> MGKYNLILSEYLSFIYNSQSAVQIPIYYSSNSELENRCIEFHSKCLENSKNGLSLRKLFVEYNDVIENATLLSILSYSYDKYNAVERKLVKYAKGKPLEADLTVNELDYENNKMTSELFPTAEEYTDSLMDPAILTSLSSNLNAVMFWLEKHENDVAEKLKVYKRRLDLFTIVASTINKYGVPRHNAKYRYEYDVMKDKPYYLVTWANSSIEMLMSVFSHDDYLIAKELIVLSYSNRSTLAKLVSSPMSILVALVDINGTFITNEELELEFSNKYVRAIVPDQTFDELNQMLDNMRKAGLVDIPKMIQDWLVDRSIEKFPLMAKIYSWSFHVGFRKQKMLDAALDQLKTEYTENVDDEMYREYTMLIRDEVVKMLEEPVKHDDHLLRDSELAGLLSMSSASNGESRQLKFGRKTIFSTKKNMHVMDDMANERYTPGIIPPVNVDKPIPLGRRDVPGRRTRIIFILPYEYFIAQHAVVEKMLIYAKHTREYAEFYSQSNQLLSYGDVTRFLSNNTMVLYTDVSQWDSSQHNTQPFRKGIIMGLDILANMTNDAKVLQTLNLYKQTQINLMDSYVQIPDGNVIKKIQYGAVASGEKQTKAANSIANLALIKTVLSRISNKHSFATKIIRVDGDDNYAVLQFNTEVTKQMIQDVSNDVRETYARMNAKVKALVSTVGIEIAKRYIAGGKIFFRAGINLLNNEKRGQSTQWDQAAILYSNYIVNRLRGFETDREFILTKIMQMTSVAITGSLRLFPSERV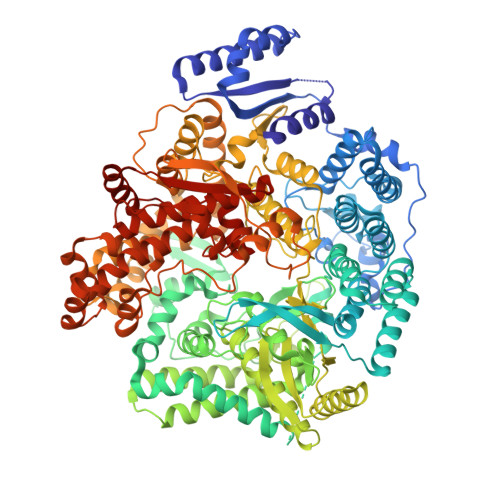LTTNSTFKVFDSEDFIIEYGTTVDEVYIQRAFMSLSSQKSGIADEIAASSTFKNYVTRLSEQLLFSKNNIVSRGIALTEKAKLNSYAPISLEKRRAQISALLTMLQKPVTFKSSKITINDILRDIKPFFTVSDAHLPIQYQKFMPTLPDNVQYIIQCIGSRTYQIEDDGSKSAISRLISKYSVYKPSIEELYKVISLHENEIQLYLISLGIPKIDADTYVGSKIYSRDKYRILESYVYNLLSINYGCYQLFDFNSPDLEKLIRIPFKGKIPAVTFILHLYAKLEVINYAIKNGSWISLFCNYPKSEMIKLWKKMWNITSLRSPYTNANFFQEPHHHHHH>[2x]MHHHHHHENLYFQSMSF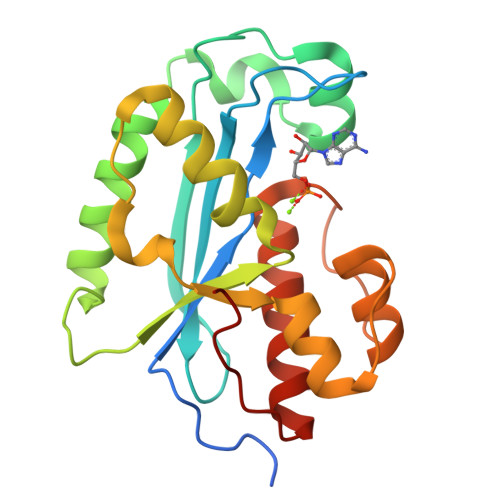PPQRYHYFLVLDFEATCDKPQIHPQEIIEFPILKLNGRTMEIESTFHMYVQPVVHPQLTPFCTELTGIIQAMVDGQPSLQQVLERVDEWMAKEGLLDPNVKSIFVTCGDWDLKVMLPGQCQYLGLPVADYFKQWINLKKAYSFAMGCWPKNGLLDMNKGLSLQHIGRPHSGIDDCKNIANIMKTLAYRGFIFKQTSKPF>SNAMISPELVKEALKKKKVRSEEAFGLEYLRFNDDYKDIPRGTAIFKDFIIWGYPHIGRIFLLETGLREQFEAPFWVEEKVDGYNTRIFKYGDNYYALSRGGFICPFTTDRLPDLIDLRILDENPDLVICAEVAGPENPYIEESPPYVKEDVQLFVFDFMKKNEQGFLSQEEKMELIEKYNLPHVEILGRFTASEEGIKKIKEILKRFNEEGREGVVFKEDSERNKRAKYITSYANLMDIKTNAKNMLQLPPEY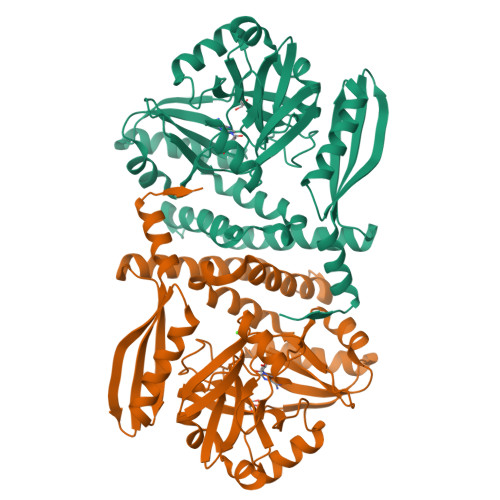YTNRILRLVLFMYEEGLKTTEHLYEELGRAFIDGLFQAIEQFEKEHKVYKTFTCKFRKKENAIALLELLSKTSKHIQVKERRLEKEGDYWRLEFDKVFLNMTGLLGHLLSGGIVYD[2x]>[2x]MGKGDVNVTSNVQAITSPQTTTIDNQTGAVTYSNWDGKVNGTVTATYNGQSYTATLNETAGKEN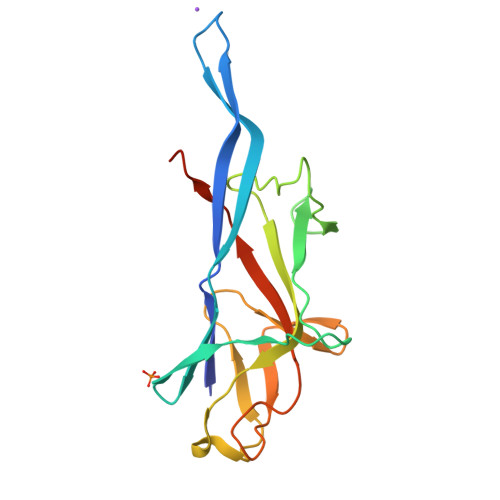SRVTPWYTQDGGKTWNVLKKDGGVYRLEPAGKYQLSVNNVSFNFGTANANKKNITLTSSNGVQFRENGQWKDSIKVSTDQNGAVSQPLTLLIPITPVDVTNAKSHHHHHH TAZOBACTAM INTERMEDIATE 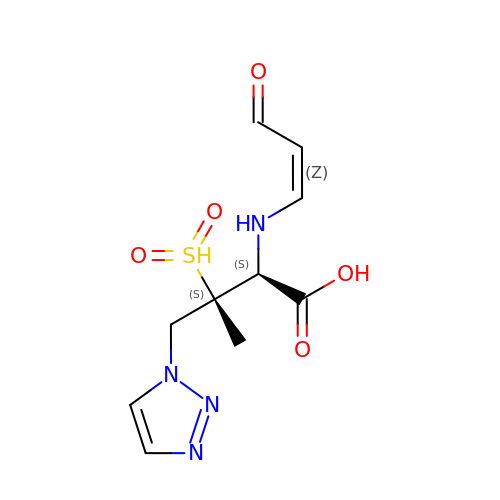| C10 H14 N4 O5 S | ANZZKUOZZHRUQC-AARLMMRRSA-N>[4x]GPLGSPEFMEASPASGPRHLMDPHIFTSNFNNGIGRHKTYL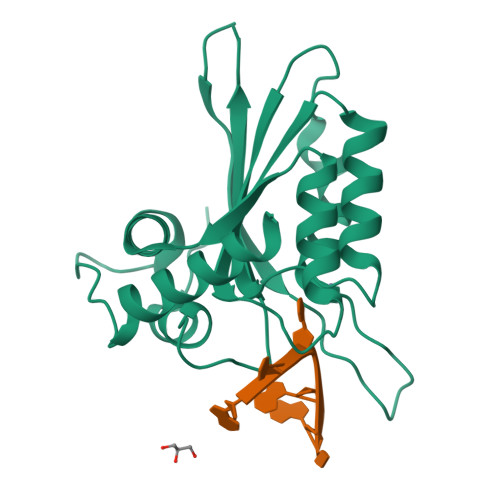CYEVERLDNGTSVKMDQHRGFLHNQAKNLLCGFYGRHAALRFLDLVPSLQLDPAQIYRVTWFISWSPCFSWGCAGEVRAFLQENTHVRLRIFAARIYDYDPLYKEALQMLRDAGAQVSIMTYDEFKHCWDTFVDHQGCPFQPWDGLDEHSQALSGRLRAILQN>[2x]RWGSMTHFSQQDNFSVAARVLGALFYYAPESAEAAPLVAVLTSDGWETQWPLPEASLAPLVTAFQTQCEETHAQAWQRLFVGPWALPSPPWGSVW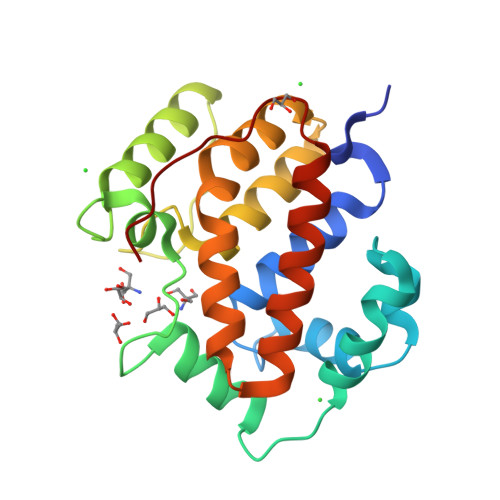LDRESVLFGDSTLALRQWMREKGIQFEMKQNEPEDHFGSLLLMAAWLAENGRQTECEELLAWHLFPWSTRFLDVFIEKAEHPFYRALGELARLTLAQWQSQLLIPVAVKPLFR>[2x]GPGSKDFQGMLEYKREDEQKLVKNLILELKPRGVAVNLIPGLPAYILFMCVRHADYLNDDQKVRSLLTSTINSIKKVLKKRGDDFE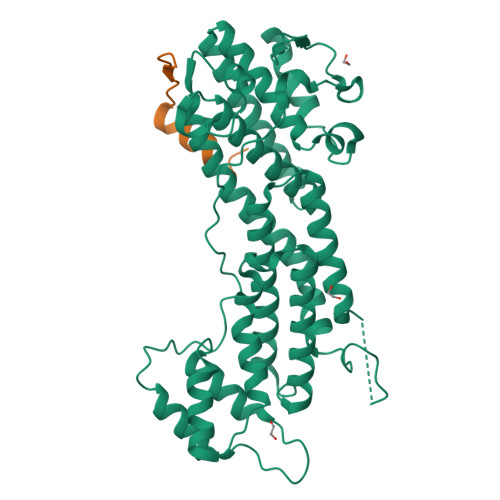TVSFWLSNTCRFLHCLKQYSGEEGFMKHNTSRQNEHCLTNFDLAEYRQVLSDLAIQIYQQLVRVLENILQPMIVSGMLEHETIQGVSGVKPTGLRKRTSSIADEGTYTLDSILRQLNSFHSVMCQHGMDPELIKQVVKQMFYIVGAITLNNLLLRKDMCSWSKGMQIRYNVSQLEEWLRDKNLMNSGAKETLEPLIQAAQLLQVKKKTDDDAEAICSMCNALTTAQIVKVLNLYTPVNEFEERVSVSFIRTIQMRLRDRKDSPQLLMDAKHIFPVTFPFNPSSLALETIQIPASLGLGFIARV;>[2x]GPGSQPTRRQIRLSSPERQRLSSLNLT>MKPEVEQELAHILLTELLAYQFASPVRWIETQDVFLKDFNTERVVEIGPSPTLAGMAQRTLKNKYESYDAALSLHREILCYSKDAKEIYYTPDPSELAAKEEPAKEEAPAPTPAASAPAPAAAAPAPVAAAAPAAAAAEIADEPVKASLLLHVLVAHKLKKSLDSIPMSKTIKDLVGGKSTVQNEILGDLGKEFGTTPEKPEETPLEELAETFQDTFSGALGKQSSSLLSRLISSKMPGGFTITVARKYLQTRWGLPSGRQDGVLLVALSNEPAARLGSEADAKAFLDSMAQKYASIVGVDLSSAASASGAAGAGAAAGAAMIDAGALEEITKDHKVLARQQLQVLARYLKMDLDNGERKFLKEKDTVAELQAQLDYLNAELGEFFVNGVATSFSRKKARTFDSSWNWAKQSLLSLYFEIIHGVLKNVDREVVSEAINIMNRSNDALIKFMEYHISNTDETKGENYQLVKTLGEQLIENCKQVLDVDPVYKDVAKPTGPKTAIDKNGNITYSEEPREKVRKLSQYVQEMALGGPITKESQPTIEEDLTRVYKAISAQADKQDISSSTRVEFEKLYSDLMKFLESSKEIDPSQTTQLAGMDVEDALDKDSTKEVASLPNKSTISKTVSSTIPRETIPFLHLRKKTPAGDWKYDRQLSSLFLDGLEKAAFNGVTFKDKYVLITGAGKGSIGAEVLQGLLQGGAKVVVTTSRFSKQVTDYYQSIYAKYGAKGSTLIVVPFNQGSKQDVEALIEFIYDTEKNGGLGWDLDAIIPFAAIPEQGIELEHIDSKSEFAHRIMLTNILRMMGCVKKQKSARGIETRPAQVILPMSPNHGTFGGDGMYSESKLSLETLFNRWHSESWANQLTVCGAIIGWTRGTGLMSANNIIAEGIEKMGVRTFSQKEMAFNLLGLLTPEVVELCQKSPVMADLNGGLQFVPELKEFTAKLRKELVETSEVRKAVSIETALEHKVVNGNSADAAYAQVEIQPRANIQLDFPELKPYKQVKQIAPAELEGLLDLERVIVVTGFAEVGPWGSARTRWEMEAFGEFSLEGCVEMAWIMGFISYHNGNLKGRPYTGWVDSKTKEPVDDKDVKAKYETSILEHSGIRLIEPELFNGYNPEKKEMIQEVIVEEDLEPFEASKETAEQFKHQHGDKVDIFEIPETGEYSVKLLKGATLYIPKALRFDRLVAGQIPTGWNAKTYGISDDIISQVDPITLFVLVSVVEAFIASGITDPYEMYKYVHVSEVGNCSGSGMGGVSALRGMFKDRFKDEPVQNDILQESFINTMSAWVNMLLISSSGPIKTPVGACATSVESVDIGVETILSGKARICIVGGYDDFQEEGSFEFGNMKATSNTLEEFEHGRTPAEMSRPATTTRNGFMEAQGAGIQIIMQADLALKMGVPIYGIVAMAATATDKIGRSVPAPGKGILTTAREHHSSVKYASPNLNMKYRKRQLVTREAQIKDWVENELEALKLEAEEIPSEDQNEFLLERTREIHNEAESQLRAAQQQWGNDFYKRDPRIAPLRGALATYGLTIDDLGVASFHGTSTKANDKNESATINEMMKHLGRSEGNPVIGVFQKFLTGHPKGAAGAWMMNGALQILNSGIIPGNRNADNVDKILEQFEYVLYPSKTLKTDGVRAVSITSFGFGQKGGQAIVVHPDYLYGAITEDRYNEYVAKVSAREKSAYKFFHNGMIYNKLFVSKEHAPYTDELEEDVYLDPLARVSKDKKSGSLTFNSKNIQSKDSYINANTIETAKMIENMTKEKVSNGGVGVDVELITSINVENDTFIERNFTPQEIEYCSAQPSVQSSFAGTWSAKEAVFKSLGVKSLGGGAALKDIEIVRVNKNAPAVELHGNAKKAAEEAGVTDVKVSISHDDLQAVAVAVSTKK[6x];>[6x]MDAYSTRPLTLSHGSLEHVLLVPTASFFIASQLQEQFNKILPEPTEGFAADDEPTTPAELVGKFLGYVSSLVEPSKVGQFDQVLNLCLTEFENCYLEGNDIHALAAKLLQENDTTLVKTKELIKNYITARIMAKRPFDKKSNSALFRAVGEGNAQLVAIFGGQGNTDDYFEELRDLYQTYHVLVGDLIKFSAETLSELIRTTLDAEKVFTQGLNILEWLENPSNTPDKDYLLSIPISCPLIGVIQLAHYVVTAKLLGFTPGELRSYLKGATGHSQGLVTAVAIAETDSWESFFVSVRKAITVLFFIGVRCYEAYPNTSLPPSILEDSLENNEGVPSPMLSISNLTQEQVQDYVNKTNSHLPAGKQVEISLVNGAKNLVVSGPPQSLYGLNLTLRKAKAPSGLDQSRIPFSERKLKFSNRFLPVASPFHSHLLVPASDLINKDLVKNNVSFNAKDIQIPVYDTFDGSDLRVLSGSISERIVDCIIRLPVKWETTTQFKATHILDFGPGGASGLGVLTHRNKDGTGVRVIVAGTLDINPDDDYGFKQEIFDVTSNGLKKNPNWLEEYHPKLIKNKSGKIFVETKFSKLIGRPPLLVPGMTPCTVSPDFVAATTNAGYTIELAGGGYFSAAGMTAAIDSVVSQIEKGSTFGINLIYVNPFMLQWGIPLIKELRSKGYPIQFLTIGAGVPSLEVASEYIETLGLKYLGLKPGSIDAISQVINIAKAHPNFPIALQWTGGRGGGHHSFEDAHTPMLQMYSKIRRHPNIMLIFGSGFGSADDTYPYLTGEWSTKFDYPPMPFDGFLFGSRVMIAKEVKTSPDAKKCIAACTGVPDDKWEQTYKKPTGGIVTVRSEMGEPIHKIATRGVMLWKEFDETIFNLPKNKLVPTLEAKRDYIISRLNADFQKPWFATVNGQARDLATMTYEEVAKRLVELMFIRSTNSWFDVTWRTFTGDFLRRVEERFTKSKTLSLIQSYSLLDKPDEAIEKVFNAYPAAREQFLNAQDIDHFLSMCQNPMQKPVPFVPVLDRRFEIFFKKDSLWQSEHLEAVVDQDVQRTCILHGPVAAQFTKVIDEPIKSIMDGIHDGHIKKLLHQYYGDDESKIPAVEYFGGESPVDVQSQVDSSSVSEDSAVFKATSSTDEESWFKALAGSEINWRHASFLCSFITQDKMFVSNPIRKVFKPSQGMVVEISNGNTSSKTVVTLSEPVQGELKPTVILKLLKENIIQMEMIENRTMDGKPVSLPLLYNFNPDNGFAPISEVMEDRNQRIKEMYWKLWIDEPFNLDFDPRDVIKGKDFEITAKEVYDFTHAVGNNCEDFVSRPDRTMLAPMDFAIVVGWRAIIKAIFPNTVDGDLLKLVHLSNGYKMIPGAKPLQVGDVVSTTAVIESVVNQPTGKIVDVVGTLSRNGKPVMEVTSSFFYRGNYTDFENTFQKTVEPVYQMHIKTSKDIAVLRSKEWFQLDDEDFDLLNKTLTFETETEVTFKNANIFSSVKCFGPIKVELPTKETVEIGIVDYEAGASHGNPVVDFLKRNGSTLEQKVNLENPIPIAVLDSYTPSTNEPYARVSGDLNPIHVSRHFASYANLPGTITHGMFSSASVRALIENWAADSVSSRVRGYTCQFVDMVLPNTALKTSIQHVGMINGRKLIKFETRNEDDVVVLTGEAEIEQPVTTFVFTGQGSQEQGMGMDLYKTSKAAQDVWNRADNHFKDTYGFSILDIVINNPVNLTIHFGGEKGKRIRENYSAMIFETIVDGKLKTEKIFKEINEHSTSYTFRSEKGLLSATQFTQPALTLMEKAAFEDLKSKGLIPADATFAGHSLGEYAALASLADVMSIESLVEVVFYRGMTMQVAVPRDELGRSNYGMIAINPGRVAASFSQEALQYVVERVGKRTGWLVEIVNYNVENQQYVAAGDLRALDTVTNVLNFIKLQKIDIIELQKSLSLEEVEGHLFEIIDEASKKSAVKPRPLKLERGFACIPLVGISVPFHSTYLMNGVKPFKSFLKKNIIKENVKVARLAGKYIPNLTAKPFQVTKEYFQDVYDLTGSEPIKEIIDNWEKYEQS

The structure of the 2.6 MDa yeast fatty acid synthase (FAS) has been studied by electron microscopy since the 1960s. The yeast fatty acid synthase (FAS) was one of the first protein complexes to be analyzed in structural biology. Yeast FAS is a prime example for revealing co-translational subunit association as a mechanism in the assembly of eukaryotic proteins. It is also critical for the production of fatty acids in microbes as a platform for chemical synthesis.

For cryoEM, the FAS sample purified as above was incubated with NADPH and malonyl-CoA prior to plunge-freezing. Although this treatment results in a slight decrease in the thermal protein stability as determined by TSA, it reduces sample heterogeneity by driving the synthesis of bound fatty acids to completion. Ser1440 is located in the dimerization module DM4 that holds the PPT domain at the perimeter of the barrel. The phosphate group is embedded in a pocket near Asp1516 and Arg1518. The two cysteines are not conserved in fungal FASs, and the density possibly originates from the malonyl group, which binds to cysteine(s) owing to the high malonyl-CoA concentration in solution. In the structure, the NADPH cofactor is bound to the active site of the KR domain [Fig. 3(d)], but not to the ER domain.>[4x]MKKGHHHHHHLVPRGSRKKIFKPEELRQALMPTLEALYRQDPESLPFRQPVDPQLLGIPDYFDIVKNPMDLSTIKRKLDTGQYQEPWQYVDDVWLMF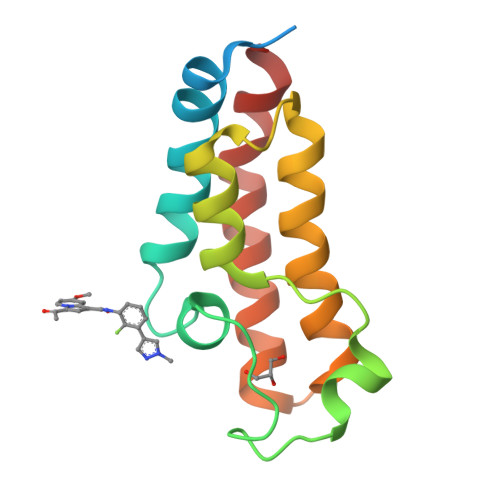NNAWLYNRKTSRVYKFCSKLAEVFEQEIDPVMQSLG>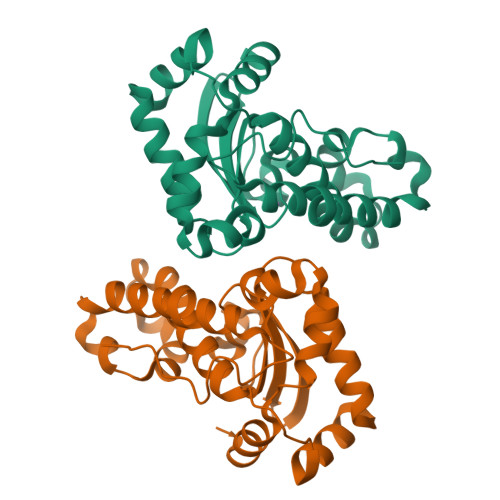[2x]SYTLPSLPYAYDALEPHFDKQTMEIHHTKHHQTYVNNANAALESLPEFANLPVEELITKLDQLPADKKTVLRNNAGGHANHSLFWKGLKKGTTLQGDLKAAIERDFGSVDNFKAEFEKAAASRFGSGWAWLVLKGDKLAVVSTANQDSPLMGEAISGASGFPIMGLDVWEHAYFLKFQNRRPDYIKEFWNVVNWDEAAARFAAKK>[10x]MSKLDLGRVDLLSMLGNSSSAGVDTAKGVIPFSTSGATWAVPRLSEDGITSHFLRRRGYVTMTQGGSRDQNAAVRKILSLIIAYDIQTQACFFISNEESMRITMAETMGVKDRPNARTNSWAEVSDSDINRGIAKALKEGNLTLDENQKDGFMKLVHAFVADILAQSGHYK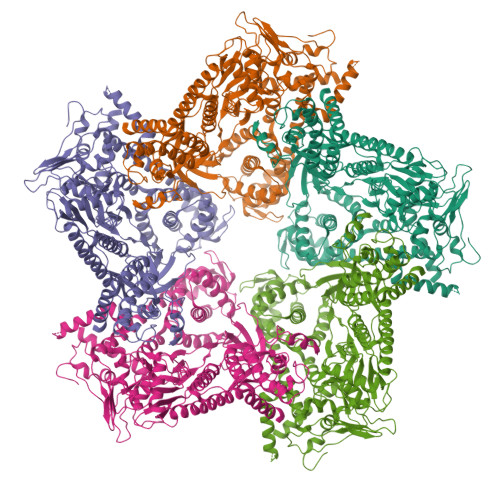PVTSVTYFSAPIDMESDYLDPFSIAIIRDVLDDSPFSELRYDARAMSELEDRDVPITRFSRVMAQMGNAMVRNIMVLNEAAQRKLRGLAVVGEIVHGRVRAPVRYLNDSFIQTLRSNINFHLLTRTTPERWAQSWIQAFGSLKGWVDAINGIADATTEEEKKKLAMQTSMDLELLSDLTPLIRDAATSVEKFVTFAPLSFYQGLGSVTQIRALDSSTNLAAVIVRYAAKEINLIPAYQSFQVPTVDVAVKKTAIMDQRLSLQLPEFSEDQFFGMLEQRMQNMSDSEVAELVDRIAKGETPFGDVVKQLPGTSTLLVTNGYYMGGLLTNEDKIIPGDASVPALLYMQAASFASSVRFPPGEYPVFHHESSNGDVRLTDQVSADAQLSHSAVETANPLNFLVACNVSVHTPSIAIDIIEPMPDLTRRGTTEYVHKGEIKVAAIPSLPPKSADRKAQVSRETAKFERVLYKARKGGAQVAAPIDLESLFGIAVNLAVPTVKHVYSPDSKTKLALDIIKGLESDGDKAAATRLLMTLARAYTGTYSSLALRRRDEITGIAAQPSDVAMQEFALQSGVQTLKAVAKHTGIMEVATIEMVEEKVRSLDDNRFYEIAAEVVLRALKGM>HHHHHHENLYFQGMAVSPSPLRIFTAGGTIDKDYRLEENGLVVGDPFVAEVLKTARLAGAVSIVALSRKDSLDFTEADREAIGRAVGQAVEDHILLTHGTDTMVETARYLGGLPELAGKTVVLSGAMVPGRVGGSDAAFNIGFACAAALMLAPGVYIAMHGKVFDPAKTRKNRGLGRFEPIDDQE[2x]

L‐Asparaginases (ASNases) catalyze the hydrolysis of L‐Asn to L‐Asp and ammonia. In contrast, the chain of ASNase from Rhodospirillum rubrum, reported here and referred to as RrA, consists of only 172 amino acid residues. RrA is homologous to the N‐terminal domain of typical bacterial class 1 ASNases and exhibits millimolar affinity for L‐Asn. Crystal structures of the wild‐type RrA, both with and without bound L‐Asp, as well as structures of several RrA mutants, reveal topologically unique tetramers.

Crystals of RrA(wt) were grown in the space group P21212, with two protomers in an asymmetric unit (a.u.). Isomorphous crystals grew both in the absence and presence of L‐Asp. In the structure of the ligand‐free enzyme, residues 58–60 of protomer A were not traced due to the lack of interpretable electron density. The two protomers form a tight dimer (designated AB in the structure) with an interface area of approximately 1100 Å2. The tetramer was created by 2‐fold crystal symmetry, with intermolecular contacts observed only between protomers A‐A' and B‐B′, yielding an interface area of around 625 Å2 for each pair. The ASFL loop is highly flexible in type II ASNases, and in the absence of a ligand in the active site it is typically disordered. However, the corresponding loop in RrA remains fully ordered regardless of the active site occupancy, and its temperature factors are comparable to those of the rest of the protein chain. Despite the overall low sequence identity between RrA and typical class 1 ASNases, here represented by EcAII, the environment of L‐Asp bound to the active site is very similar for both enzymes. As previously mentioned, Thr16 (presumed to be the primary nucleophile in RrA) remains well ordered even in the absence of a substrate.>[6x]ALFDRLGRVVRANLNDLVSKAEDPEKVLEQAVIDMQEDLVQLRQAVARTIAEEKRTEQRLNQDTQEAKKWEDRAKLALTNGEENLAREALAR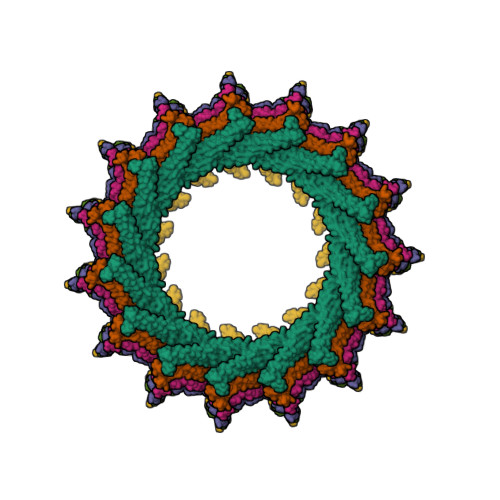KKSLTDTAAAYQTQLAQQRTMSENLRRNLAALEAKISEAKTKKNMLQARAKAAKANAELQQTLGGLGTSSATSAFERMENKVLDMEATSQAAGELAGFGIENQFAQLEASSGVEDELAALKASMAGGALPGTSAATPQLEAAPVDSSVPANNASQDDAVIDQELDDLRRRLNNL>SGTVTFDITNISHKAIDIILKVVLGIAEHEGTEVTFHSERGQLQIEVKNLHEEDKRLIEQAIEAARLADSPDPESVARAVELLTKVAKASTNTELIQFIVKELLELARKLTDPKDLAKVLDSISELLTELALKTGDPTAALAAMVAHIAELVVRLALMAERTHPGSEIVKKAVKLVQEVAEEVLEAAQLMLEKPNSDEVAKKLEEVAKKAIEACIELQQILEAWAKERGDQDLLREVREHKLQILTIAVAYKAAQMGVTVLKHTHGWVVF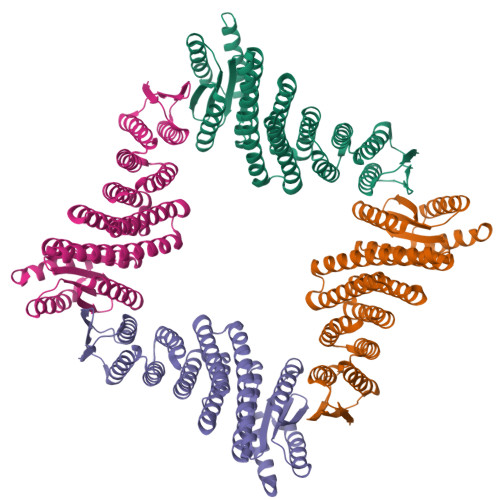LVILGLHKQQAEQLLRFVHRVAHALGVTLSITFSGDIVVIAVTVGASEEEKKEVRKIVKEIAKQLRHAETEEEAKEIVQRVIEEWQEEGGSG[4x]We verified that the Mimivirus and M. chilensis predicted PAPs were able to perform polyadenylation. These proteins were not only active, but also intrinsically self-processive, generating >700 nucleotides long polyA tails. To elucidate the molecular basis of this processivity we determined the Mimivirus and M. chilensis PAP crystallographic 3D structures, which revealed two topologically identical subdomains with a nucleotidyltransferase fold. Thus, while other PAPs form heterodimers with processivity factors, the Mimivirus and M. chilensis PAP become processive upon homodimerization.

The Mimivirus R341 and M. chilensis Mg561 genes were reliably predicted to encode PAPs after two iterations of PSI-BLAST. The Mimivirus R341 protein exhibits a unique acidic extension of 65 residues at its C-terminal end (D5) and an insertion of 12 amino acids in its third subdomain (D3). The canonical acidic residues D94-E96-D143 are properly positioned and ordered in the crystal structure as evidenced by the 2Fo-Fc electron density maps contoured at 1σ on the of M. chilensis and Mimivirus PAP active sites. To further characterize the molecular determinants of the dimerization of Mg561 and the role of the dimerization on the polyadenylation activity, we made deletion of the Mg561 (ΔD1 Mg561) and R341 (ΔD1 R341) N-terminal domains. Gel filtration experiments revealed that the mutants were monomeric and although they still co-purified with RNA, they were inactive, suggesting that the dimeric state and the N-terminal domain were required for the polyadenylation activity. No association was observed between Mg18 and R341 confirming the specificity of the interaction.

>[2x]MLKNKTRAEKYQTYYTTNEYQIVKEKLPDIIRDAEIKASEVLEPTIYEKRAIMEVIKDFIRDHQRKVYGGTALNEALKQVNPKDAIYDNYSFSDIEFYSPTPVQDLVDLCNILYRKGYKFVQGKDAQHEETYSIFVNFQLYCDITYSPTRVFYGIKTIEIDGINYTDPHFMLIDYLRMVNQPLTAAGQRWEKAFERMYRLLKDYPIEDFDKRLDIPEPPEEIQSYISRIKTEFLSDNKLNESFLISGIEAYNFYIRHAASSKDEEQMARTNRNVVNLNNFIANVPFSELISVNYREDVKNTYNFLRMIVEDKEKISVDEYFPLFQFTGYSTVIKYDDHPIIRIYEGDGYCIPNVKTVKTVENDNGTKTKYEYKYVSFQYVLMILYINKFRAHLDKNKPMYFNYGIAISNLVKARNIYLDQTGKSVLDNTVFKEFRTNCTGNTISFTRMNRLRLLEKRKQGKQTSFVYTPEDFFKKDLETQAKLDPSKARFKNTSGNKIMVPKYLLFKIDNNGNIEDNIHSEEAEISEKEETSGGSSISTDKSFEESPNSSPNSSPNNSLNNSIDISTNNYDDRSENSLDSLTSD> GSAAASPAWMPAYACQRPTPLTHHNTGLSEALEILAEAAGFEGSEGRLLTFCRAASVLKALPSPVTTLSQLQGLPHFGEHSSRVVQELLEHGVCEEVERVRRSERYQTMKLFTQIFGVGV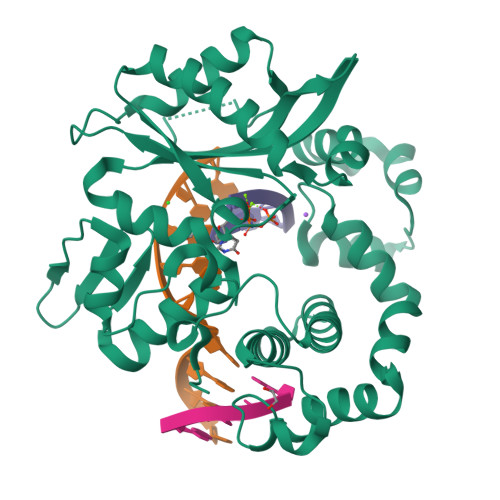KTADRWYREGLRTLDDLREQPQKLTQQQKAGLQHHQDLSTPVLRSDVDALQQVVEEAVGQALPGATVTLTGGFRRGKLQGHDVDFLITHPKEGQEAGLLPRVMCRLQDQGLILYHQHQHSCCESPTRLAQQSHMDAFERSFCIFRLPQPGSWKAVRVDLVVAPVSQFPFALLGHTGSKLFQRELRRFSRKEKGLWLNSHGLFDPEQKTFFQAASEEDIFRHLGLEYLPPEQRNA>QTCSTSDDADDPTPPNERDDEAFASRVAAAKRELEGTGTVCQINNGETDLAAKFHKSLPHD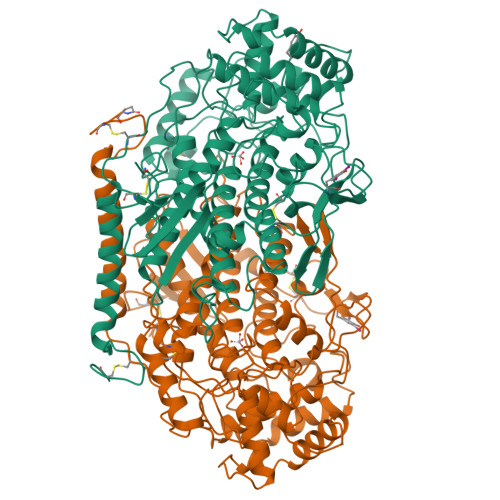DLGQVDADAFAALEDCILNGDLSICEDVPVGNSEGDPVGRLVNPTAAFAIDISGPAFSATTIPPVPTLPSPELAAQLAEVYWMALARDVPFMQYGTDDITVTAAANLAGMEGFPNLDAVSIGSDGTVDPLSQLFRATFVGVETGPFISQLLVNSFTIDSITVEPKQETFAPDVNYMVDFDEWLNIQNGGPPAGPELLDDELRFVRNARDLARVTFTDNINTEAYRGALILLGLDAFNRAGVNGPFIDIDRQAGFVNFGISHYFRLIGAAELAQRSSWYQKWQVHRFARPEALGGTLHLTIKGELNADFDLSLLENAELLKRVAAINAAQNPNNEVTYLLPQAIQEGSPTHPSYPSGHATQNGAFATVLKALIGLDRGGDCYPDPVYPDDDGLKLIDFRGSCLTFEGEINKLAVNVAFGRQMLGIHYRFDGIQGLLLGETITVRTLHQELMTFAEESTFEFRLFTGEVIKLFQDGTFTIDGFKCPGLVYTGVENCV[2x]>MASMTGGQQMGRGSMNEPIGEPGRSPASDTAEKAQAIAAARNTFARDNPVSAGHHERARRSMPGGNTRSILFHRPFPLVIAQGTGSRFQDVDGHAYVNFLGEYTAGLFGHSHPVIRAAVERALAVGLNLSTQTENEALFAEAVCDRFPSIDLVRFTNSGTEANLMALATATAITGRKTVLAFDGGYHGGLLNFASGHAPTNAPYHVVLGVYNDVEGTADLLKRHGHDCAAILVEPMLGAGGCVPAERAFLDLLRAEASRCGALLIFDEVMTSRLSGGGAQEMLGISADLTTLGKYIGGGMSFGAFGGRRDLMERFDPARDGAFAHAGTFNNNILTMSAGHAALTQIYTRQAASDLSASGDRFRANLNRIAVENQAPLQFTGLGSLGTIHFSRAPIRSAGDVRAADQQLKELFFFHMLRKGIYLAPRGMYALSLEIADAGRDAFAEALADFIGEQRALLMAAALEH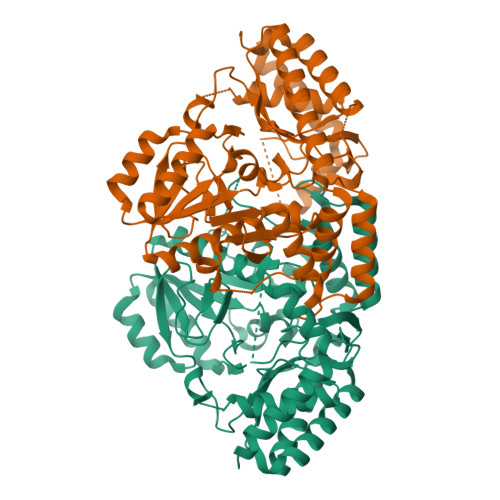HHHHH[2x]>MLRREFGPKYTAKINEAEENWQARAEAIKKGKKQNTW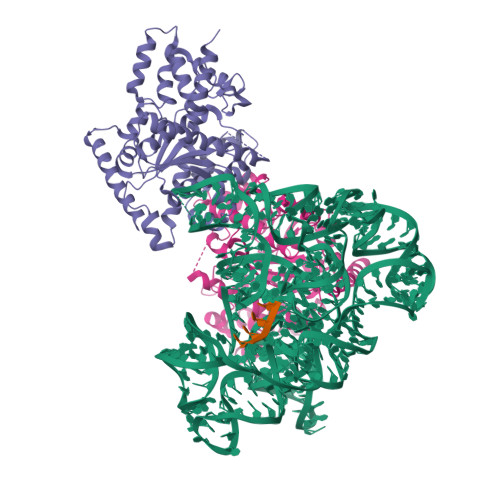DLFEERGYVKDTAGTKEHIAELMRTRRIGAYVGIDPTAPSLHVGHLLPLMPLFWMYLEGYKAFTLIGGSTAKIGDPTGRLKSRDHLSSSDATMNMTKIHYQLKKLWENVDTQMRARGYEADWARKRGIVNNNHWWNKQPMLEVLRRVGHALRIGPMLSRDTVKNKMTQGDGVSFAEFTYPIMQGWDWFELFYQQGVQMQIGGSDQYGNIISGLEVVKAARESEPDPQERKYVTPKTALDECVGFTVPLLTDSSGAKFGKSAGNAIWLDPYQTSVFDFYGYFVRRSDQEVENLLKLFTFMPISEITKTMEEHIKDPSKRVAQHTLAREVVTLVHGKQEASAAEDQHRMMYTGQMTI[8x]>MHHHHHHEKNITVTASVDPVIDLLQADGNALPSAVKLAYSPASKTFESYRVMTQVHTNDATKKVIVKLADTPQLTDVLNSTVQMPISVSWGGQVLSTTAKEFEAAALGYSASGVNGVSSSQEL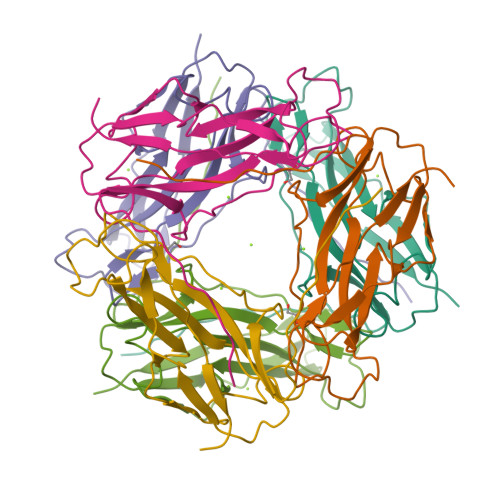VISAAPKTAGTAPTAGNYSGVVSLVMTLGS[3x]In the first step of the HP, GFAT synthesizes d-glucosamine-6-phosphate (GlcN6P) from l-glutamine (l-Gln) and Frc6P, releasing l-glutamate (l-Glu). GFAT contains two domains: the glutaminase domain responsible for releasing ammonia in the hydrolysis of l-Gln to l-Glu and the isomerase/transferase domain, which catalyzes both the isomerization of Frc6P to d-glucose-6-phosphate (Glc6P) as well as the transfer of ammonia to Glc6P to produce GlcN6P. The active sites of the two domains are linked by an ammonia channel, which forms when GFAT engages with both of its substrates, l-Gln and Frc6P. The main distinctive feature between prokaryotic and eukaryotic GFAT is the feedback inhibition by the HP product UDP-GlcNAc, which inhibits the glutaminase function.

We wondered how the presence of l-Glu and GlcN6P would affect the structure and co-crystallized GFAT-1 in the presence of both product molecules. The GlcN6P-bound structure formed the same asymmetric dimer as the Glc6P-bound structure and a linear sugar was present in the active site. Compared to human GFAT-1, the GlcN6P-bound E. coli structure shows the pyranose ring GlcN6P in the active site and no electron density for the glutaminase domain is observed, although the full-length protein was crystallized. While in the E. coli structure the product might have already left the active site, destabilizing the glutaminase domain, our structure represents the last step of catalysis, just before departure of the GlcN6P product.

>MCGIFAYLNYHVPRTRREILETLIKGLQRLEYRGYDSAGVGFDGGNDKDWEANACKIQLIKKKGKVKALDEEVHKQQDMDLDIEFDVHLGIAHTRWATHGEPSPVNSHPQRSDKNNEFIVIHNGIITNYKDLKKFLESKGYDFESETDTETIAKLVKYMYDNRESQDTSFTTLVERVIQQLEGAFALVFKSVHFPGQAVGTRRGSPLLIGVRSEHKLSTDHIPILYRTGKDKKGSCNLSRVDSTTCLFPVEEKAVEYYFASDASAVIEHTNRVIFLEDDDVAAVVDGRLSIHRIKRTAGHHHHHHDHPGRAVQTLQMELQQIMKGNFSSFMQKEIFEQPESVVNTMRGRVNFDDYTVNLGGLKDHIKEIQRCRRLILIACGTSYHAGVATRQVLEELTELPVMVELASDFLDRNTPVFRDDVCFFLSQSGETADTLMGLRYCKERGALTVGITNTVGSSISRETDCGVHINAGPEIGVASTKAYTSQFVSLVMFALMMCDDRISMQERRKEIMLGLKRLPDLIKEVLSMDDEIQKLATELYHQKSVLIMGRGYHYATCLEGALKIKEITYMHSEGILAGELKHGPLALVDKLMPVIMIIMRDHTYAKCQNALQQVVARQGRPVVICDKEDTETIKNTKRTIKVPHSVDCLQGILSVIPLQLLAFHLAVLRGYDVDFPRNLAKSVTVE[2x]>[10x]M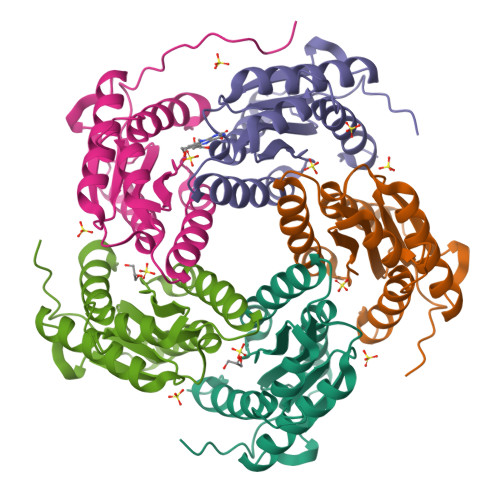RGSHHHHHHGSAVKGLGQLDQNYDGSKLRVGIIHARWNRVIIDALVKGAIDRMLSLGVKEENIIVETVPGSFELPYGSKRFAEKQAKKGEPLDVVIPIGVLIKGSTMHFEYISDSTTQAIMNLQDKINIPVIFGLLTCLTEEQALARAGIDEGKTMHNHGEDWGAAAVEMATKFGANA5-(ACETYLAMINO)-3,5-DIDEOXY-2-O-PHOSPHONO-D-ERYTHRO-L-MANNO-NONONIC 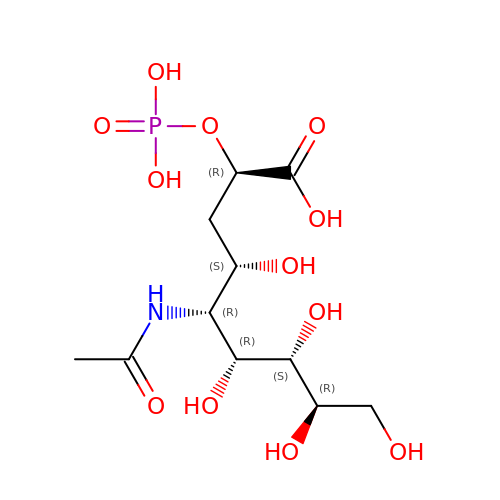ACID | C11 H22 N O12 P | SQZISPQQTAMDAM-IHICSVBISA-N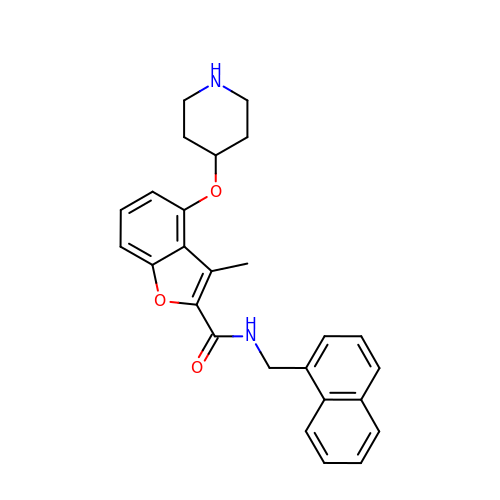3-methyl-N-(naphthalen-1-ylmethyl)-4-piperidin-4-yloxy-1-benzofuran-2-carboxamide | C26 H26 N2 O3 | JDZKIYVLMLQBQF-UHFFFAOYSA-N> SGVDDDMACHKIPVEADFLYAYSTAPGYYSWRNSKDGSWFIQSLCAMLKQYADKLEFMHILTRVNRKVATEFESFSFDATFHAKKQIPCIVSMLTKELYF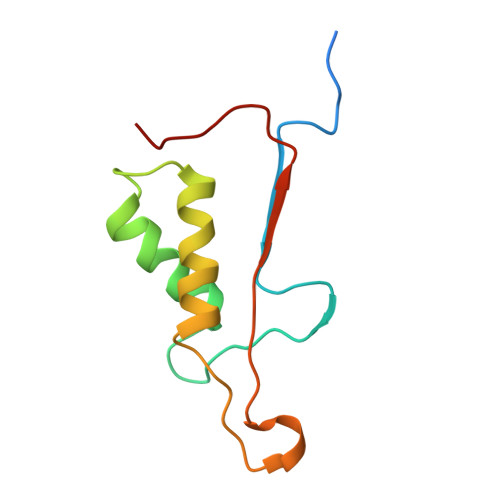YH> EPPADGGQIKGVGSGRCLDVPDASTSDGTQLQLWDCHSGTNQQWAATDAGELRVYGDKCLDAAGTSNGSKVQIYSCWGGDNQKWRLNSDGSVVGVQSGLCLDAVGNGTANGTLIQL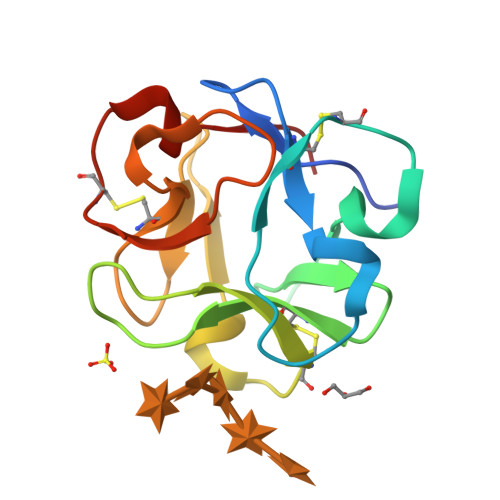YTCSNGSNQRWTRT3-(3-hydroxyphenyl)-1~{H}-pyrrolo[3,4-g]indol-8-one | C16 H10 N2 O2 | 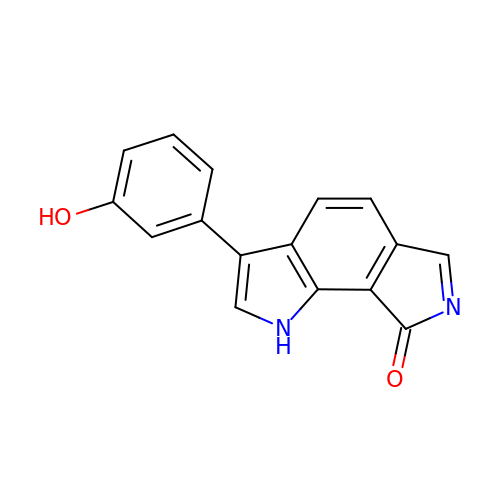NIESWLNGCVKLAW-UHFFFAOYSA-N The final step involves the insertion of iron into sirohydrochlorin and is catalysed by a sirohydrochlorin ferrochelatases. Here we have confirmed our hypothesis that cbiX, sometimes but not always found adjacent to nir operon, is not primarily a cobaltochelatase but rather the missing terminal enzyme of siroheme synthesis in many denitrifying bacteria. Our protein, Pp-CbiX represents the first sirohydrochlorin ferrochelatase structure. However, our in vivo functional data has demonstrated that Pp-CbiX acts as a ferrochelatase, by acting to insert iron into the tetrapyrrole substrate in preference to cobalt ion.

In addition, with this purified sample, crystals were grown and the crystal structure of Pp-CbiX was determined to a resolution of 1.9 Å. The overall structure of Pp-CbiX is characteristic of the type II class of metal chelatase enzymes. A search of the PBD using PDBeFold (EMBL-EBI) showed that the full length Pp-CbiX protein is most similar to CbiK from Salmonella enterica, a cobaltochelatase (Se-CbiK). Splitting the structure in this way identified the most similar structure to the Pp-CT domain as the CbiXS protein from Archaeoglobus fulgidus (Af-CbiXs, with a metallated sirohydrochlorin bound), with an RMSD of 1.88 Å. The structural overlay shows the metallated tetrapyrrole fits into the central cavity in Pp-CbiX and indicates that the active site residues in Pp-CbiX are located in the CT half of the protein, similar to Se-CbiK but unlike CbiXL and SirB that have active site residues in their NT. The overlay highlights the conserved position in the active site of the (His127) residue of Pp-CbiX with the equivalent His residue in Se-CbiK (His145), shown to be involved in metal binding in the bound tetrapyrrole. The functional importance of (His127) from Pp-CbiX was demonstrated by mutating this residue to alanine, which resulted in the loss of in vivo ferrochelatase activity of Pp-CbiXH127A. Mutagenesis of (His187) in our protein demonstrated that this residue was indeed essential for the ferrochelatase activity of Pp-CbiX. Interestingly, in the structure of Pp-CbiX, the functionally essential (His187) points away from the active site of the enzyme. So it is feasible that (His187) of Pp-CbiX is also at a very flexible region of the structure, and this crystal form has captured the (His187) residue in an inactive conformation in which it is moved out of the way of the active site.

> MVRNVLIVAHGQPGDPAPQQRAIEALAARVAPLVPQACVRGATLAMPGALDRADDETLIYPLFMATGWFTRSELPRRLALAGAPKARILPPFGSDPGLPALCLALIAQAAETQGWPLAGTRLLVAAHGSGRSRAPSEAARRIAAGLAPYAAAATCGFIEEAPFIADAARDLPERAICLPLFATQAEHVTDDLPAALSQAGFQGLVLPPVGLAPQVPAMIAESIKAALSKRP> ANPLYQKHIISINDLSRDDLNLVLATAAKLKANPQPELLKHKVIASCFFEASTRTRLSFETSMHRLGASVVGFSDSANTSLGKKGETLADTISVISTYVDAIVMRHPQEGAARLATEFSGNVPVLNAGDGSNQHPTQTLLDLFTIQETQGRLDNLHVAMVGDLKFGRTVHS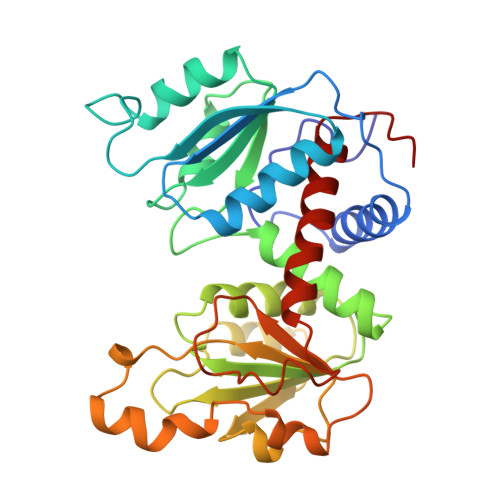LTQALAKFDGNRFYFIAPDALAMPQYILDMLDEKGIAWSLHSSIEEVMAEVDILYMTRVQKERLDPSEYANVKAQFVLRASDLHNAKANMKVLHPLPRVDEIATDVDKTPHAWYFQQAGNGIFARQALLALVLNRDLVL The gene encoding for ChiP is found in most marine members of the Vibrionaceae, emphasizing the general importance of this OM diffusion channel for chitin utilization. The addition of micromolar concentrations of chitooligosaccharides such as chitohexaose (GlcNAc6) causes a complete block of ionic current, demonstrating tight binding. Here, we report X-ray crystal structures of VhChiP in the absence and presence of chitooligosaccharides.

We expressed VhChiP without a His-tag in the OM of the porin-deficient E. coli Bl21 omp8 strain and obtained reasonable yields (~3 mg from 12 l of culture) even though VhChiP overexpression appeared to be highly toxic for E. coli. The purified protein was crystallized in the presence of 0.4% C8E4 as detergent. The obtained crystals of VhChiP in space group C2 diffracted to reasonable resolutions of ~2.5 Å. The crystal structure of the OM-expressed channel is almost identical to that of the in vitro-folded protein. Strikingly however, in OM-expressed VhChiP the N-termini plug the pore of a neighboring β-barrel within the trimeric assembly, effectively blocking all β-barrels for substrate transport. The reason that the plug is inter- and not intra-molecular might be due to fact that the N-terminal β-strand is pointing away from its own pore towards the neighboring one. All residues of the N-terminus have good electron density in the structure and a number of polar interactions can be identified between the N-terminal plug and the barrel, most notably between Asp1 (carboxylate)-Arg94/148, Asp1 (α-amino group)-Y118/Asp122, Ala3-Glu53, Asn4-Asn127/Arg312/Glu347, Ser5-Asp122, Asp6-Arg94, and Lys9-Glu76. Thus, five out of the first six residues of the N-terminus make polar interactions with the pore of the protein, suggesting that the plug is stably inserted in the pore. As expected from the interactions observed in the crystal structure, the plug in natively expressed VhChiP is very stable with root mean square fluctuations (RMSF) of about 1.5 Å.

>[3x]DGANSDAAKEYLTKDSFSYEVYGIIAMQAAYRDYDSGDAKQDDNLGGMQLNNESRIGFRGKKQFANFEPTFIWQIEGGYVDPSFGGEGAGLGERDTFVGFESASWGQVRLGRVLTPMYELVDWPASNPGLGDVYDWGGAIGGAKYQDRQSNTIRWDSPMYADKFSIDAAVGAGDKAGLGAGDDYWGGIAAHYKLGPLQLDAAYEGNRNIEAEGQTWENNTYLVGVQGWFENGISFFAQYKYMEADASNGVNEKQDAMSAGLMYTTGDWQYKLGYAANFDLERDGKTLSNTSDDVVSAQIMYFVDPSAVLYARARMNDFNEGLDGLDDAARWTSGTNGDYNEYSVGVEYYF> LQRLHMLQISYFRDPYHVWYQGNASLGGHLTHVLEGPDTNTTIIQLQPLQEPESWARTQSGLQSYLLQFHGLVRLVHQERTLAFPLTIRCFLGCELPPEG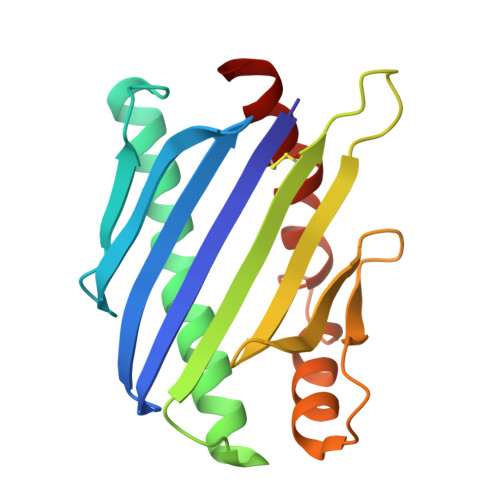SRAHVFFEVAVNGSSFVSFRPERALWQADTQVTSGVVTFTLQQLNAYNRTRYELREFLEDTCVQYVQKHI1-[(3-thiophen-3-ylphenyl)methyl]-3~{H}-pyrrol-2-one | C15 H13 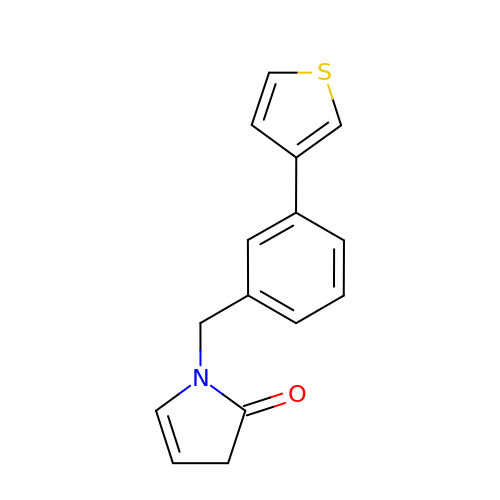N O S | DMVGEVMEROXRGX-UHFFFAOYSA-N>[2x]MEKILIFGHQNPDTDTICSAIAYADLKNKLGFNAEPVRLGQVNGETQYALDYFKQESPRLVETAANEVNGVILVDHNERQQSIKDIEEVQVLEVIDHQRIANFETAEPLYYRAEPVGCTATILNKMYKENNVKI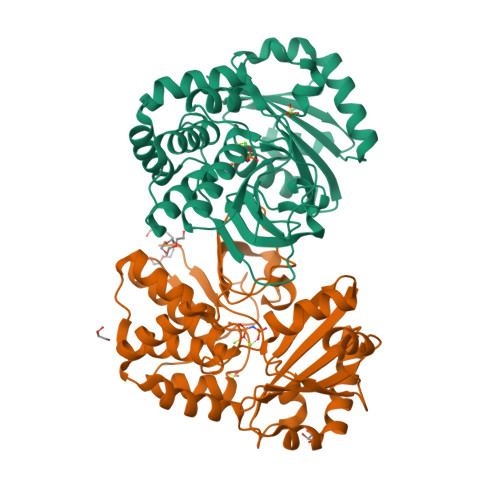EKEIAGLMLSAIISDSLLFKSPTCTDQDVAAAKELAEIAGVDAEEYGLNMLKAGADLSKKTVEELISLDAKEFTLGSKKVEIAQVNTVDIEDVKKRQAELEAVISKVVAEKNLDLFLLVITDILENDSLALAIGNEAAKVEKAFNVTLENNTALLKGVVSRKKQVVPVLTDAMAE>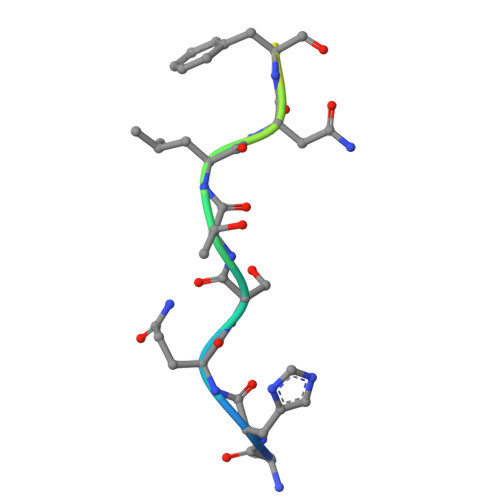 KHQSTLNFKHRVTKP>GVTLLLPEPEWTYPRLSCPGSTFQKALLISPHRFGETKGNSAPLIIREPFIACGPKECKHFALTHYAAQPGGYYNGTRGDRNKLRHLISVKLGKIPTVENSIFHMAAWSGSACHDGKEWTYIGVDGPDNNALLKIKYGEAYTDTYHSYANNILRTQESACNCIGGNCYLMITDGSASGISECRFLKIREGRIIKEIFPTGRVKHTEECTCGFASNKTIECACRD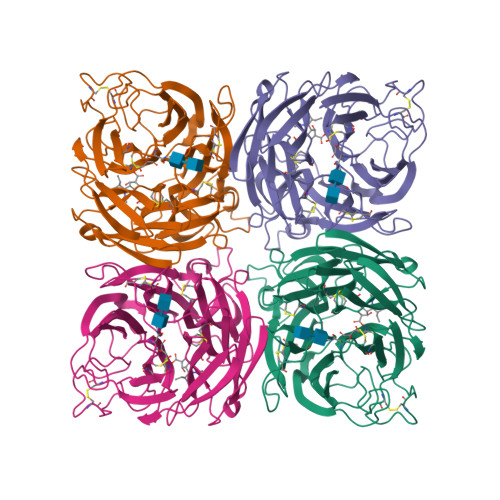NSYTAKRPFVKLNVETDTAEIRLMCTETYLDTPRPDDGSITGPCESNGDKGSGGIKGGFVHQRMASKIGRWYSRTMSKTKRMGMGLYVKYDGDPWTDSDALALSGVMVSMEEPGWYSFGFEIKDKKCDVPCIGIEMVHDGGKETWHSAATAIYCLMGSGQLLWDTVTGVDMAL[2x]> MITIVVIPTAHFSWTDTNFLNSVDYRLTSQPKIRDRFAVYAPGWLRRQLDEFSASLTASELLQALQTIPIPVKARCLLLPKPKRFAQWLLDVPSANIWHIPVTTLRATVASKHPSSDVYNYIPDHVPPNAEFDTVTRRVAAGRDIYVRSTKVIGAPLCLAAPAKYYAGYLSTHQLDGIYPENWAPDNFHKREFCLTILPSLLGPRTFLLDVDADRDASYPLSVLWPQLRALALKSRLLLPPVALLRRVVDPGLKPTWSADSDAAFRALRLSRPSSASKPVGFDFSALPVVDIICLLESEPDDHGRIAPGTRLTIHSVPTDLLTSLSIQEGVRYPLRQESGMFVHWVLLALLMSDDVTISGTRRSVKLETAHASARPFVHITVERCASARIIDVRGSPAMYANAVCLTLPKGSYKSTIIDTLPAMFSDLPILEQAAVIDSDALGDSLRPSFETQFLERLENLDPNLLDRAVASILSPTSDTSDDAVTTVLDAFNALYREIMTPAQRARLPLLTQQGRVLAFAHSDYELLSANIPIQVVRGSIPIDHVVNLLARRNRVGGTAL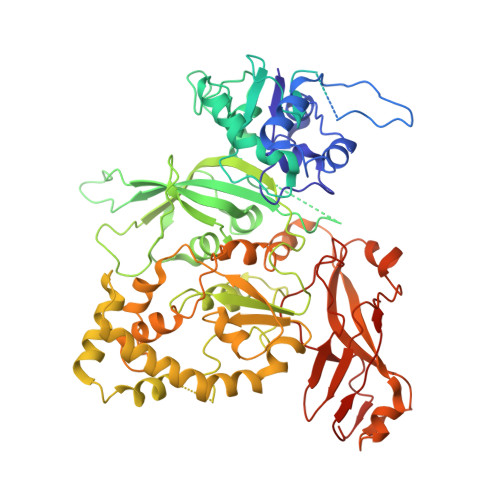QVLLDYCYRTQASPLAPTPAGRLYKQLFGPWLMVPRLSEPLIKLRLVASAPAKVLRAAGWTIDGDPPLEVSCLCAYVTDRAAATALIERRLDSRALVTVGGDQLMFVEYAPPLPLVSIPRTFLLPVTYVVHWVPPQRVLLNGGNVSFTSGLEWTFDDDPQVVTSTGV> KRAHHNALERKRRDHIKDSFHSLRDSVPSLQGEKASRAQILDKATEYIQYMRRKNHTHQQDIDDLKRQN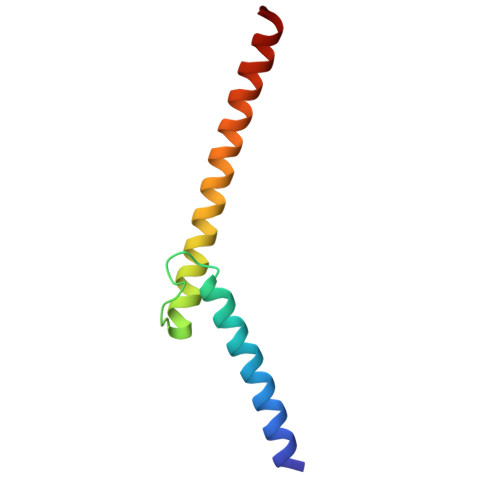ALLEQQV N-[(1S,2R)-2-hydroxy-1-(hydroxycarbamoyl)propyl]-4-[4-(phenylethynyl)phenyl]piperidine-1-carboxamide 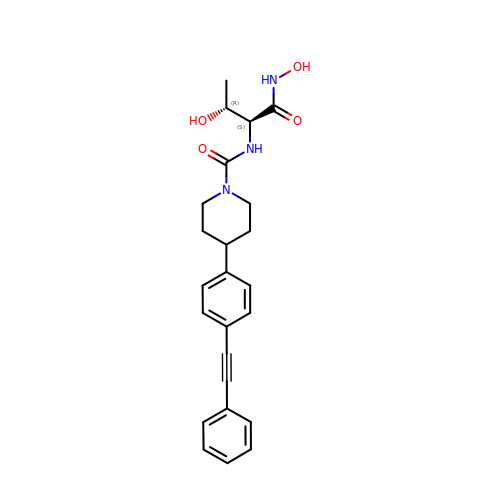| C24 H27 N3 O4 | SRSVRACVPWREJZ-VGSWGCGISA-N>MKKLLVKELIEQFQDCVNLIDGHTNTSNVIRVPGLKRVVFEMLGLFSSQIGSVAILGKREFGFLSQKTLVEQQQILHNLLKLNPPAIILTKSFTDPTVLLQVNQTYQVPILKTDFFSTELSFTVETYINEQFATVAQIHGVLLEVFGVGVLLTGRSGIGKSECALDLINKNHLFVGDDAIEIYRLGNRLFGRAQEVAKKFMEIRGLGIINVERFYGLQITKQRTEIQLMVNLLSLEKQTTVTFERLGTELKKQRLLGVDLSFYEIPISPGRKTSEIIESAVIDFKLKHSGYNSALDFIENQKAILKRKKDES[6x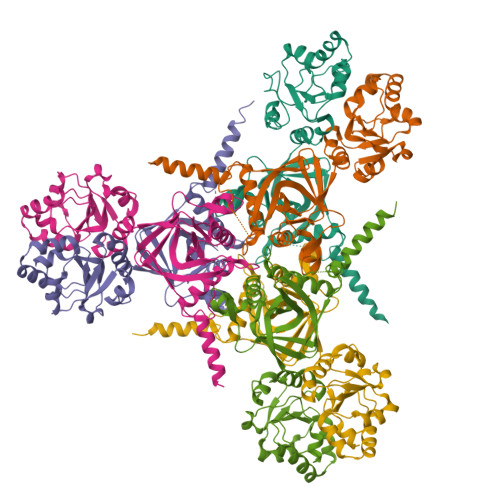]1-{1-[2-(methylsulfonyl)phenyl]-7-propoxyindolizin-3-yl}ethanone 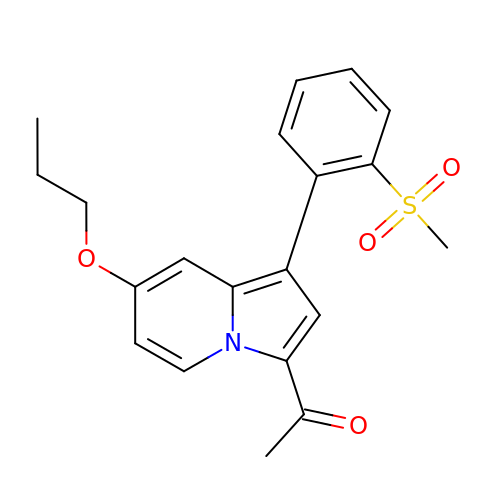| C20 H21 N O4 S | KHWCPNJRJCNVRI-UHFFFAOYSA-N> GPHMLESHQQTDEIARSLKIFAQVT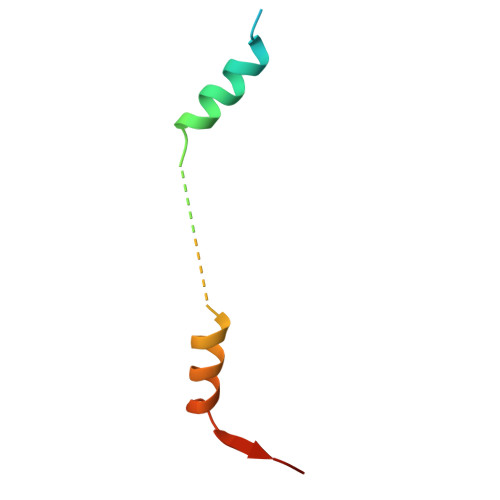TGAAENAAGSMQDVMQEFATNGYASDDLG[(2~{S},5~{R})-1-[(2~{R},3~{S},4~{R},5~{R})-5-(6-aminopurin-9-yl)-3,4-bis(oxidanyl)oxolan-2-yl]-5-azaniumyl-6-oxidanyl-6-oxidanylidene-hexan-2-yl]-(2-methylpropyl)azanium 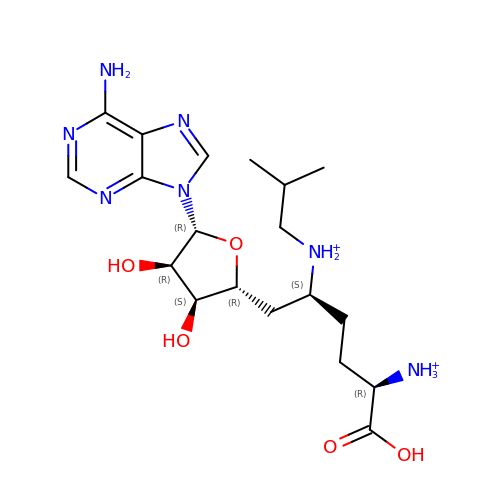| C19 H33 N7 O5 | JFKLCPCUECHESR-SNDYUSLUSA-P> DSLGREAKCYNELNGCTKIYDPVCGTDGNTYPNECVLCFENRKRQTSILIQ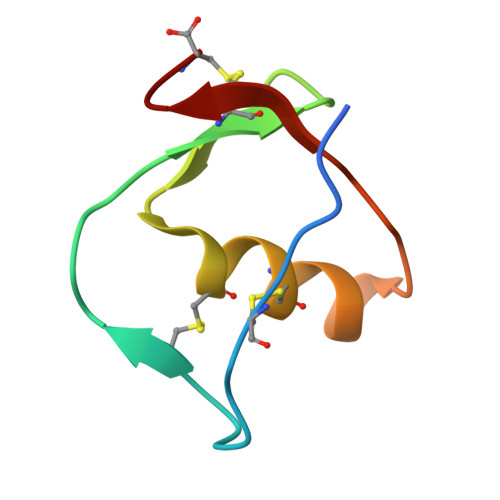KSGPC> GSHMGTRDDEYDYLFKVVLIGDSGVGKSNLLSRFTRNEFNLESKSTIGVEFATRSIQVDGKTIKAQIWDTAGLERYRAITSAYYRGAVGALLVYDIAKHLTYENVERWLKELRDHADSNIVIMLVGNKSDLRHLRAVPTDEARAFAEKNGLSFIETSALDSTNVEAAFQTILTEIYRIVSQKQMSDRRENDMSPSNNVVPIHVPPTTENKPKVQCCQNI;> GSHMQNNSAKQSWLLRLFESKLFDISMAISYLYNSKEPGVQAYIGNRLFCFRNEDVDFYLPQLLNMYIHMDEDVGDAIKPYIVHRCRQSINFSLQCALLLGAYSSDMHISTQRHSRGTKLRKLILSDELKPANLKRTAANPKVENEDEPVRLAPEREFIKSLMAIGKRLATLPTKEQKTQRLISELSLLNHKLPARVWLPTAGFDHHVVRVPHTQAVVLNSKDKAPYLIYVEVLECENFDTTSVPARIPENRRDPEDPSAVALKEPWQEKVRRIREGSPYGHLPNWRLLSVIVKCGDDLRQELLAFQVLKQLQSIWEQERVPLWIKPYKILVISADSGMIEPVVNAVSIHQVKKQSQLSLLDYFLQEHGSYTTEAFLSAQRNFVQSCAGYCLVCYLLQVKDRHNGNILLDAEGHIIHIDFGFILSSSPRNLGFETSAFKLTTEFVDVMGGLDGDMFNYYKMLMLQGLIAARKHMDKVVQIVEIMQQGSQLPCFHGSSTIRNLKERFHMSMTEEQLQLLVEQMVDGSMRS

In this article, we describe an application of hydrogen deuterium exchange mass spectrometry (HDX‐MS) to identify dynamic regions within type III phosphatidylinositol 4 kinase beta (PI4KIIIβ) in complex with the GTPase Rab11. All deletions were then combined into a single construct that contained two internal deletions, as well as removing the N‐terminus and the C‐terminus. This construct, referred to from now on as xtalPI4K (HsPI4KB S294A 121–784, Δ249–287, Δ408–507), enabled us to generate crystals of PI4KIIIβ in complex with Rab11.

Using HDX‐MS to identify disordered regions and map conformational changes in the kinase PI4KIIIβ bound to the small GTPase Rab11 allowed us to successfully crystallize this complex in the presence of both GTPγS and GDP loaded forms of Rab11 and to collect data to resolutions of 2.65 and 3.2 Å, respectively. This approach also permitted us to generate crystals of PI4KIIIβ in the absence of small molecule inhibitors, enabling us to soak these crystals with the potent PI4K inhibitor BQR695, and solve the cocrystal structure with this compound. The hydrogen bond between V598 and the central quinoxaline is characteristic of many protein and lipid kinase inhibitors, as this mimics the hydrogen bond made with the N1 of the ATP adenine. This compound has been shown to be specific over PI3K kinases (10 fold more potent against PI4KIIIβ relative to p110α, and >100 fold more potent against PI4KIIIβ compared with all other class I and class III PI3K isoforms). PI4KIIIβ has a larger binding pocket to accommodate the glycyl methyl amide group compared to the class I and class III PI3Ks. The wall of this pocket is composed of L383 in PI4KIIIβ, which corresponds to a tryptophan in class I PI3Ks, and a phenylalanine in class III PI3Ks [Fig. 7(D,E)]. The clash at this position is likely to interfere with the ability of the central quinoxaline of BQR695 to properly hydrogen bond with V598 of PI4KIIIβ.>[2x]MENSIEAYLAD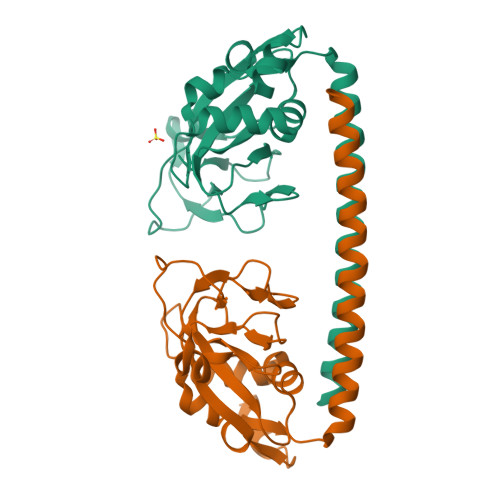SREKVTLGTVVDCFKGKAVSSKVVPGDVGLINLSDMGTLGIQYHQLRTFQMDRRQLLRYLLEDGDVLIASKGTLKKVCVFHKQNRDVVASSNITVLRPQKLLRGYYIKFFLDSPIGQALLDAADHGKDVINLSTKELLDIPIPVIPLVKQDYLINHYLRGLTDYHRKLNRAEQEWEYIQNEIQKGLGLEHHHHHH Here, we report that a critical glycine residue (Gly463) dominates the motion of threonyl-tRNA synthetase (ThrRS) and the sensitivity of the enzyme to antibiotics. The natural product Obafluorin (OB) is a potent inhibitor of bacterial threonyl-tRNA synthetase (ThrRS). Our previous work showed that OB covalently binds to ThrRS, forming an ester bond with a tyrosine residue in the catalytic center via the highly strained β-lactone ring, making OB the first covalent aaRS inhibitor with demonstrated crystal structures. The binding of OB induces a large conformational change in ThrRS.

In the apo state EcThrRS_G463S structure, the sidechain of the highly conserved residue Gln484 in the catalytic pocket forms a hydrogen bond with Tyr462, while in the OB-bound structure of the wild type (open state), the conformation of Gln484 is changed to accommodate OB. The distance between Ser463 and the conformation-altered Gln484 is only 1.6 Å. To test the possibility that Ser463 might become resistant to OB by blocking the conformational change of Gln484, we designed a G463S_Q484A mutant to remove the sidechain of Gln484 to avoid potential spatial conflicts. However, in the TSA experiment, OB increased the Tm of EcThrRS_G463S_Q484A by 17.2 °C, 10 °C less than the effect of 36j, suggesting that the EcThrRS_G463S_Q484A mutant, similar to EcThrRS_G463S, could still not be covalently inhibited by OB. Consistently, cocrystallizing 300 μM EcThrRS_G463S_Q484A protein with 600 μM OB did not yield an EcThrRS_G463S_Q484A–OB complex structure. The EcThrRS_G463S_Q484A structure is still in an apo state. Therefore, G463S endows ThrRS with resistance to OB neither by altering the protein’s structure nor by direct or indirect spatial repulsion.

>[2x]MRDHRKIGKQLDLYHMQEEAPGMVFWHNDGWTIFRELEVFVRSKLKEYQYQEVKGPFMMDRVLWEKTGHWDNYKDAMFTTSSENREYCIKPMNCPGHVQIFNQGLKSYRDLPLRMAEFGSCHRNEPSGSLHGLMRVRGFTQDDAHIFCTEEQIRDEVNGCIRLVYDMYSTFGFEKIVVKLSTRPEKRIGSDEMWDRAEADLAVALEENNIPFEYQLGEGAFYSPKIEFTLYDCLDRAWQCGTVALDFSLPSRLSASYVGEDNERKVPVMIHRAILGSMERFIGILTEEFAGFFPTWLAPVQVVIMNITDSQSEYVNELTQKLSNAGIRVKADLRNEKIGFKIREHTLRRVPYMLVCGDKEVESGKVAVRTRRGKDLGSMDVNEVIEKLQQEIRSRSLKQLEELEHHHHHH> GPMVSKSDQLLIVVSILEGRHFPKRPKHMLVVEAKFDGEQLATDPVDHTDQPEFATELAWEIDRKALHQHRLQRTPIALQCFALDPVTSAKETIGYIVLDLRTAQETKQAPKWYQLLSNKYT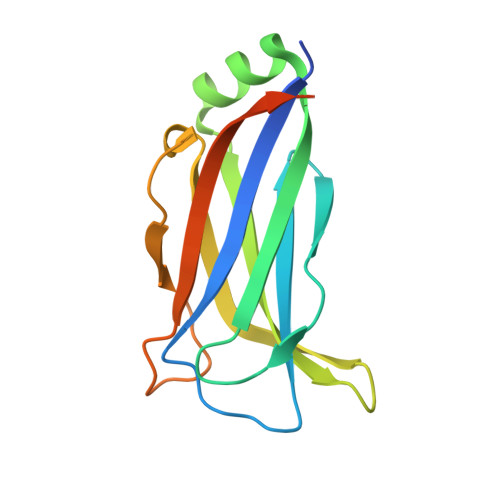KFKSEIQISIALETDTKPPVDSFKAKGAPPR> QTLCDQYATYSNGRYTVYNNLWGKSSGSGSQCTYVDSIS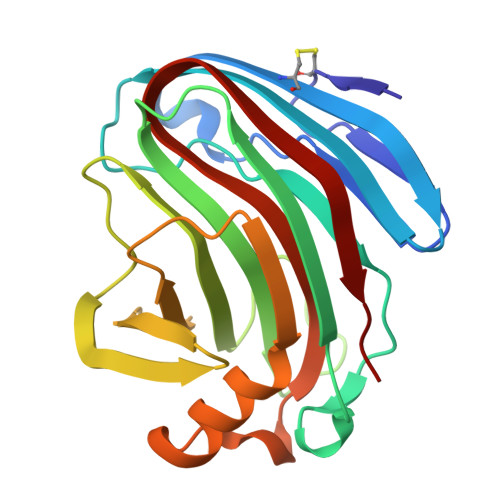NSGVAWHTTWTWSGGDNQVKSYANSQVSLTKKLVSQISSIPTTVQWSYDNTNTRADVAYDLFTAADINHVTYSGDYELMIWLARYGSVQPIGSQIDSVNIGGHTWELWYGGSTQKTYSFVSATPITSFSGDVMDFWDYLTSRHGYPASSQYLINMQFGTEPFTGGPATLRVSQWTASVN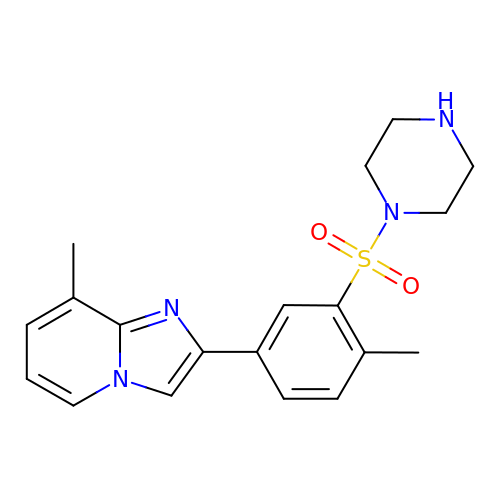8-methyl-2-(4-methyl-3-piperazin-1-ylsulfonyl-phenyl)imidazo[1,2-a]pyridine | C19 H22 N4 O2 S | VEQQFFCWFKIQSW-UHFFFAOYSA-N>MQKYALHAYPVMALMVATLTGCAWIPAKPLVQGATTAQPIPGPVPVANGSIFQSAQPINYGYQPLFEDRRPRNIGDTLTIVLQENVSASKSSSANASRDGKTSFGFDTVPRYLQGLFGNSRADMEASGGNSFNGKGGANASNTFSGTLTVTVDQVLANGNLHVVGEKQIAINQGTEFIRFSGVVNPRTISGSNSVPSTQVADARIEYVGNGYINEAQNMGWLQRFFLNLSPM[26x];>MFKALAGIVLALVATLAHAERIRDLTSVQGVRENSLIGYGLVVGLDGTGDQTTQTPFTTQTLNNMLSQLGITVPTGTNMQLKNVAAVMVTASYPPFARQGQTIDVVVSSMGNAKSLRGGTLLMTPLKGVDSQVYALAQGNILVGGAGASAGGSSVQVNQLNGGRITNGAIIERELPTQFGAGNTINLQLNDEDFTMAQQITDAIN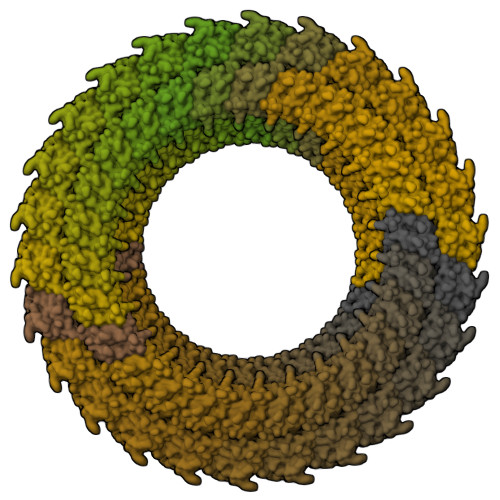RARGYGSATALDARTVQVRVPSGNSSQVRFLADIQNMEVNVTPQDAKVVINSRTGSVVMNREVTLDSCAVAQGNLSVTVNRQLNVNQPNTPFGGGQTVVTPQTQIDLRQSGGSLQSVRSSANLNSVVRALNALGATPMDLMSILQSMQSAGCLRAKLEII[26x]> MSPIIEANGTLDELTSFIGEAKHYVD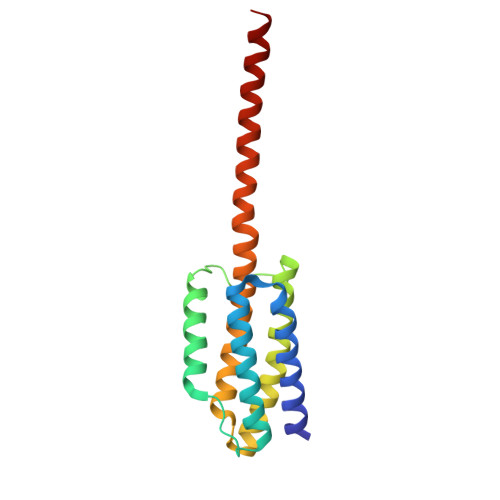EEMKGILEEIQNDIYKIMGEIGSKGKIEGISEERIKWLEGLISRYEEMVNLKSFVLPGGTLESAKLDVCRTIARRAERKVATVLREFGIGKEALVYLNRLSDLLFLLARVIEIAAAAQLEKELQALEKENAQLEWELQALEKELAQ>GHMGFFSRDIQTMEDLLLHGLRDIYYAEQQITKA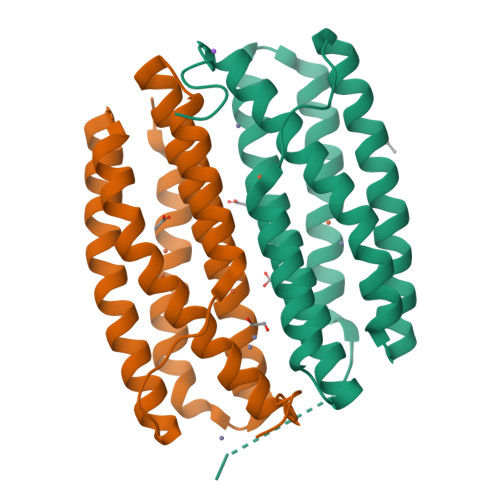LPKMIEQATNRDLSQGLTSHLEETQKQIERLDQVFKKLGQKPSGVNCPAIDGLIKEADETAGEIADKTVLDAAIVANAQAVEHYEIARYGTLIAWAEELGHDDIVRFLTTNLNEEKAANTKLNTVALRKGVNRKAASGS[2x]>[2x]MASMTGGQQMGRGSMSRDPLPFFPPLYLGGPEITTENCEREPIHIPGSIQPHGALLTADGHSGEVLQ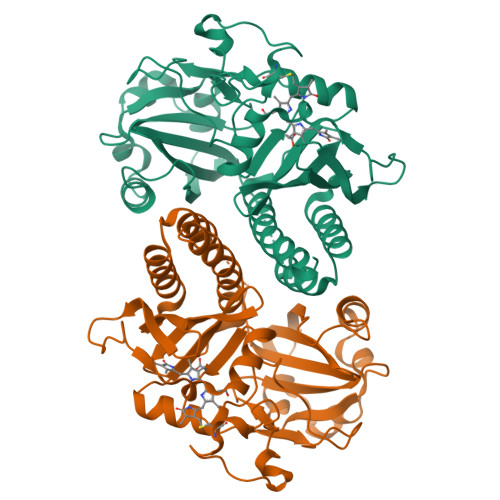MSLNAATFLGQEPTVLRGQTLAALLPEQWPALQAALPPGCPDALQYRATLDWPAAGHLSLTVHRVGELLILEFEPTEAWDSTGPHALRNAMFALESAPNLRALAEVATQTVRELTGFDRVMLYKFAPDATGEVIAEARREGLHAFLGHRFPASDIPAQARALYTRHLLRLTADTRAAAVPLDPVLNPQTNAPTPLGGAVLRATSPMHMQYLRNMGVGSSLSVSVVVGGQLWGLIACHHQTPYVLPPDLRTTLEYLGRLLSLQVQVKEALEHHHHHH The mammalian antibacterial protein siderocalin (Scn), also known as lipocalin 2 (Lcn2), neutrophil gelatinase-associated lipocalin (NGAL) or 24p3, functions by sequestering iron as bacterial siderophore complexes. Scn tightly binds a variety of bacterial siderophores including many catechol-based compounds from enteric bacteria, such as enterobactin (Ent; equilibrium dissociation constant (KD)  = 0.4±0.1 nM), but does not bind many hydroxamate-based siderophores, such as desferrioxamine (DFO). Iron transport by Scn requires the presence of a siderophore, since Scn has no measurable affinity for iron alone. The importance of Scn in antibacterial defense was demonstrated with Scn knock-out mice, which are profoundly susceptible to bacterial infections.

Since Fe(catechol)x complexes were readily observed binding in the Scn calyx by crystallography, Scn was co-crystallized in the presence of Fe(2,3-DHBA)3 and a 1∶3 mixture of iron and GA to mimic the 2,3-DHBA co-crystallization conditions. The Scn/Fe(2,3-DHBA)3 structure showed clear electron density for three 2,3-DHBA groups and bound iron in the calyx, while the Scn/Fe/GA structure showed only weak electron density features in the calyx consistent with water molecules and the unresolved side-chain of W79, despite ≥millimolar concentrations of protein and GA in the crystallization mix. For mixtures of iron and 2,3-DHBA, the Fe:L complex was predominant in solution and was successfully modeled in an association equilibrium with Scn (KD = 0.101±0.002 nM); the interaction between Scn and desferri 2,3-DHBA was more than a thousand-fold weaker (KD = 0.40±0.01 µM). At neutral pH, Ent and 2,3-DHBA chelate ferric ions in solution through the adjacent catechol 2-and 3-OH groups, generating complete, hexadentate FeEnt complexes or incomplete Fe(2,3-DHBA)x complexes. As the pH is lowered, iron binding shifts from catecholate-mode to salicylate-mode, engaging the 2-OH and carbonyl oxygens, and then to iron release. The shift from catecholate-to salicylate-mode binding is accompanied by an outward swing of the catechol groups, widening the ferric complex to a diameter that is also sterically incompatible with two of three pockets in the rigid calyx of Scn. Scn generally crystallizes at pHs in the 4 to 4.5 range. While this is below the release pH for catechol complexes, a partially-released complex was observed because of the high concentration of components and the very non-physiological conditions in the crystallization trials. Bacterial catecholate siderophores, like Ent and its substituent, 2,3-dihydroxybenzoic acid (2,3-DHBA), are unlikely to fulfill the requirements of an iron delivery pathway because iron is not released from Scn/siderophore/iron complexes (holo-Scn) until acidification below pH 4, which is not readily achieved in most cellular compartments, such as endocytic vesicles.

>MPLGLLWLGLALLGALHAQAQDSTSDLIPAPPLSKVPLQQNFQDNQFQGKWYVVGLAGNAILREDKDPQKMYATIYELKEDKSYNVTSVLFRKKKCDYWIRTFVPGSQPGEFTLGNIKSYPGLTSYLVRVVSTNYNQHAMVFFKKVSQNREYFKITLYGRTKELTSELKENFIRFSKSLGLPENHIVFPVPIDQCIDG[4x]>[12x]LELT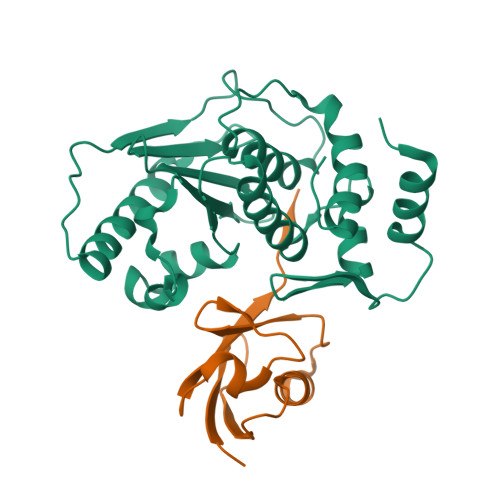EDMEKEISNALGHGPQDEILSSAFKLRITRGDIQTLKNYHWLNDEVINFYMNLLVERNKKQGYPALHVFSTFFYPKLKSGGYQAVKRWTKGVNLFEQEIILVPIHRKVHWSLVVIDLRKKCLKYLDSMGQKGHRICEILLQYLQDESKTKRNSDLNLLEWTHHSMKPHEIPQQLNGSDSGMFTCKYADYISRDKPITFTQHQMPLFRKKMVWEILHQQLL;>[12x]EYIKLKVIGQDSSEIHFKVKMTTHLKKLMESYCQRQGVPMNSLRFLWEGQRIADNHTPKELGMEEEDVIEVYQEQTGG>MDRRRFIKGSMAMAAVCGTSGIASLFSQAAFAADSDIADGQTQRFDFSILQSMAHDLAQTAWRGAPRPLPDTLATMTPQAYNSIQYDAEKSLWHNVENRQLDAQFFHMGMGFRRRVRMFSVDPATHLAREIHFRPELFKYNDAGVDTKQLEGQSDLGFAGFRVFKAPELARRDVVSFLGASYFRAVDDTYQYGLSARGLAIDTYTDSKEEFPDFTAFWFDTVKPGATTFTVYALLDSASITGAYKFTIHCEKSQVIMDVENHLYARKDIKQLGIAPMTSMFSCGTNERRMCDTIHPQIHDSDRLSMWRGNGEWICRPLNNPQKLQFNAYTDNNPKGFGLLQLDRDFSHYQDIMGWYNKRPSLWVEPRNKWGKGTIGLMEIPTTGETLNNIVCFWQPEKAVKAGDEFAFQYRLYWSAQPPVHCPLARVMATRTGMGGFSEGWAPGEHYPEKWARRFAVDFVGGDLKAAAPKGIEPVITLSSGEAKQIEILYIEPIDGYRIQFDWYPTSDSTDPVDMRMYLRCQGDAISETWLYQYFPPAPDKRQYVDDRVMSLEHH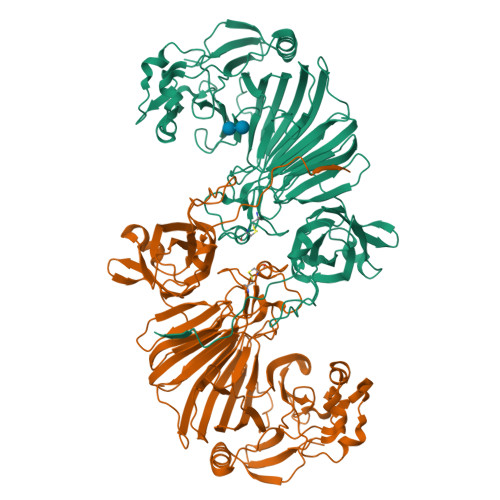HHHH[12x]>MMDKFRMIFQFLQSNQESFMNGICGIMALASAQMYSAFDFNCPCLPGYNAAYSAGILLAPPLVLFLLGLVMNNNVSMLAEEWKRPPGRRAKDPAVLRYMFCSMAQRALWAPVVWVAVTLLDGKCFLCAFCTAVPVSALGNGSLAPGLPAPELARLLARVPCPEIYDGDWLLAREVAVRYLRCISQALGWSFVLLTTLLAFVVRSVRPCFTQAAFLKSKYWSHYIDIERKLFDETCTEHAKAFAKVCIQQFFEAMNHDLELGHTNGTLA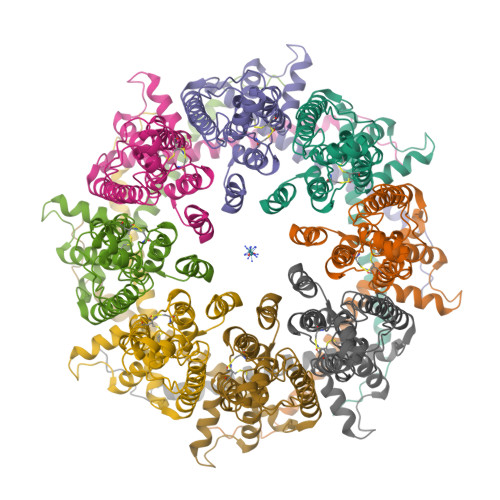TAPASAAAPTTPDGAEEEREKLRGITDQGTMNRLLGSAWSHPQFEK[8x]Important for NTHi survival, colonization and persistence in vivo is the Sap (sensitivity to antimicrobial peptides) ABC transporter system. An essential system for NTHi survival and persistence in vivo is the Sap (sensitivity to antimicrobial peptides) transporter. This multi-component system uses a periplasmic protein (SapA) to bind and deliver substrates to the heterodimeric inner membrane-associated Sap permease (SapBC). The Sap ABC transporter is completed by two membrane-associated nucleotide-binding proteins (SapD & SapF) that hydrolyze ATP to provide energy for substrate transport across the bacterial inner membrane. The structure confirmed the classification of SapA into the Substrate Binding Protein (SBP) superfamily, as was predicted from sequence analysis.

Hemin was also soaked into SapA crystals. As with SapAclosed, SapAheme displayed difference density in the central ligand binding pocket. However, the pocket remains too small (approximately 400 Å3) to accommodate a substantial ligand such as heme, which occupies a volume closer to 800 Å3. Furthermore, additional difference density, corresponding to heme, was present on the protein surface. The bound heme forms a crystal contact between two symmetry-related SapA molecules, each coordinating the ligand via a surface exposed histidine (His 306 in both cases). Although the heme bound in the SapAheme crystal structure is present at a crystal contact, providing a stoichiometry of 0.5, there are no further interactions between the protein molecules. Therefore, there is no reasonable basis to suggest that the 2 SapA:1 heme complex shown in Fig 5B is a physiologically relevant dimer. In addition to native gel and ITC evidence we provide structural evidence for heme binding on the surface of the SapA molecule. This surface location is far from the ligand binding cavity and out of the context of any defined pocket and may therefore cast some doubt on the physiological relevance of this interaction. Nevertheless, at the very minimum, we can conclude that a surface residue His 306 has the capacity to coordinate heme to the SapA molecule. It is the first molecular-detail experimental structural evidence for heme binding to SapA or indeed any Cluster C SBP.

> GLTYCTHASGFSFNPQTADAGTSMNVVTEQIYNKLFDIKNHSATLTPMLAQSYSISADGKEILLNLRHGVKFHQTPWFTPTRDFNAEDVVFSINRVLGHNTYLPTLAEANVTYSNPQYKVFHEQARKVRFPYFDSIKLNEKIKSVTALSPYQVKIELFAPDSSILSHLASQYAIIFSQEYAYQLSADDNLAQLDTHPVGTGPYQVKDYVYNQYVRLVRNENYWKKEAKIEHIIVDLSTDRSGRLVKFFNNECQIASYPEVSQIGLLKNDDKHYYMQSTDGMNLAYLAFNFDKPLMRDHEIRAAISQSLNRARIIHSIYHNTATVANNIIPEVSWASTVNTPEFEFDYHPKIAKNKLADKNLLLNLWVINEEQVYNPAPFKMAEMIKWDLAQAGVKVKVRAVTRPFLTAQLRNQLENYDLILSGWLAGNLDPDGFMRPILSCGTKNELTNLSNWCNEEFDQFMDRAITTSHLSSRAKAYNEAQELVLRELPIIPIANVKRILVANSRVKGVKMTPFGSLDFSTLYFI> MRTFFVGGNWKANPKTVEEAEKLIEMLNGAKVEGNVEVVVAAPFAFLPTLQQKLRKDWKVSAENVFTKPNGAFTGEVTVPMIKSFGIEWTILGHSERRDILKEDDEFLAAKAKFALENGMKIIYCCGEHLSEREAGKASEFVSAQIEKMIPAIPAGKWDDVVIAYEP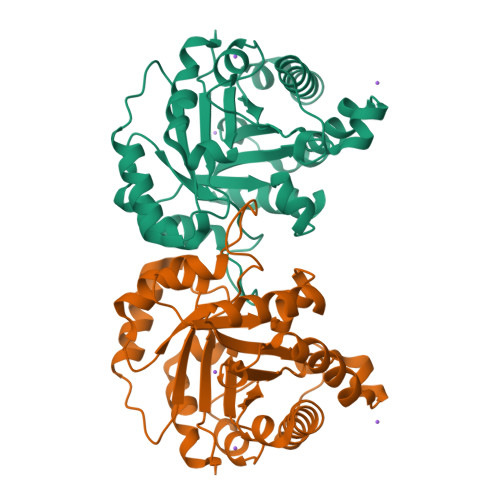IWAIGTGKVASTQDAQEMCKVIRDILAAKVGADIANKVRILYGGSVKPNNCNELAACPDVDGFLVGGASLEPGFINIVNSNVHSK~{N}-[(4-chlorophenyl)methyl]quinazolin-4-amine 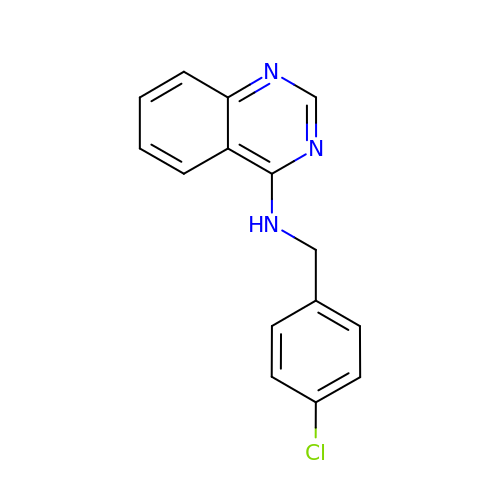| C15 H12 Cl N3 | BTRLSAYDVSPYCS-UHFFFAOYSA-N>MSQQVTQLNPTQQTTQSAFLATTVITAQCHAILNTQFTPPTVKPDWFDDLSKKLDSAKLVAKQWIDDLGPQVSASIPSSVINFDATFQASIDAIHELYKADPTASGKDNTTVQQASQIMTALSSQVSGIEATVKGMNKELSDWGVKMQAAHDDLVNGATNIQKTIIDLQTDIESMNNAIDNNRAAIEKLNKDLVYAQVAVGVGIFMLVAGVALTVATAGTAAAVS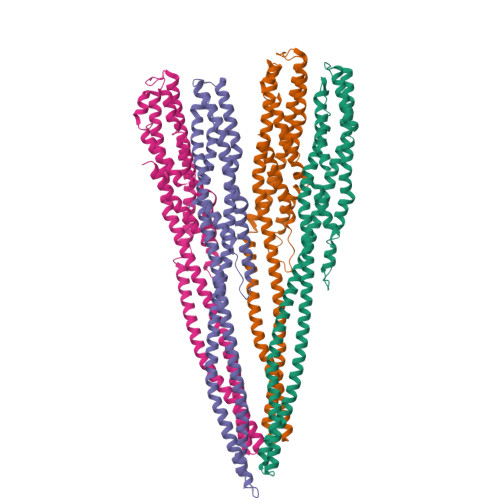GGIAAVGAASIIAGGVTWGVLQNQIDDDYDSIAQEQKQKAEDQQQIIALQGLSNASSAVVSAIETSTSVLSDFETTWTVFGNELDDVVTKLNNGASMQSIIMEKVMSDAAKNEWDDAVELAKQLASAKIAIETKELAPAVKQAA[4x]>MSKIFLKGKAIIAMLLVIAVLAFAGCSGSSTKNSSTNGNKKQVVLTLWYPWAGPDGDAVVSLAKEYSKTHPNVQIKAQMVSGAGIAATQGGGQGKFLSAVAAGNPPDLVLYWGQDALPGLADQGAIIPLDDYLKDVDTSKFFEAAYNAMKYKGKIYGLPEMVNVRVLFWNKDLFKQAGLDPNTPPKTIAELDQMAAKLTKTKNGTIEQMGFIPWIGQGVPHVMAGVFGTSLVDSNGNPILSPDKNPQLLNLLKWEVSYSDKYGAMNINKFIAGMSQNSSQANDPFVLGKVAMMISGEWQINANKQYNPKLNFGVGPIPQAPGGKPMPSLMDGNTWMIPKGSKHPQEAMDFIKWTMDPQRIADTADKVYNIAPIV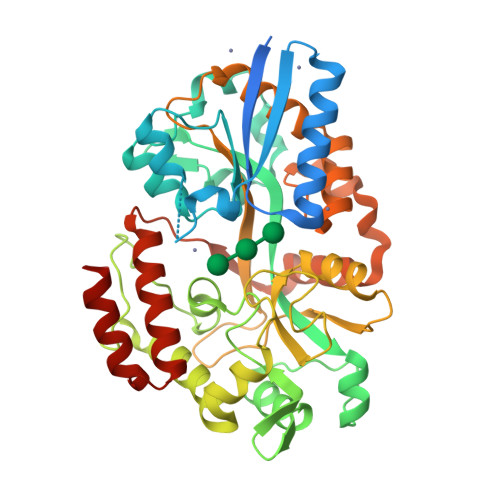EAAKIQKLNNDPYFKEVLNVAQKGSIYYTPAAKGMLSTETAANNAFQAAQYKKSTPEQALKNAQAEAEKSLSQ[2x]> LLVVGPKFIRANQEYTLVISNFNSQLSKVDLLLKLEGETDNGLSVLNVTKMVDVRRNMNRMINFNMPEDLTAGNYKITIDGQRGFSFHKEAELVYLSKSISGLIQVDKPVFKPGDTVNFRVIVLDTELKPPARVKSVYVTIRDPQRNV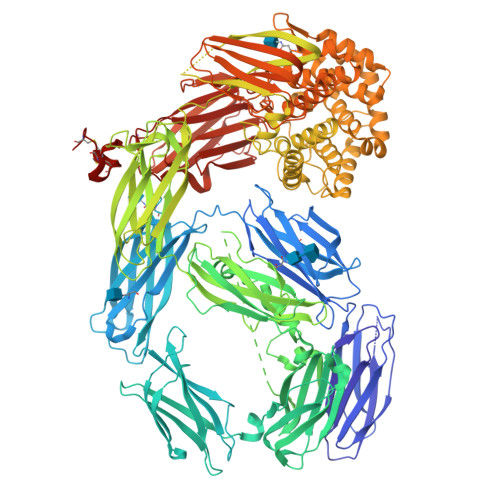IRKWSTAKLYAGVFESDLQIAPTPMLGVWNISVEVEGEELVSKTFEVKEYVLSTFDVQVMPSVIPLEEHQAVNLTIEANYHFGKPVQGVAKVELYLDDDKLKLKKELTVYGKGQVELRFDNFAMDADQQDVPVKVSFVEQYTNRTVVKQSQITVYRYAYRVELIKESPQFRPGLPFKCALQFTHHDGTPAKGISGKVEVSDVRFETTTTSDNDGLIKLELQPSEGTEQLSIHFNAVDGFFFYEDVNKVETVTDAYIKLELKSPIKRNKLMRFMVTCTERMTFFVYYVMSKGNIIDAGFMRPNKQPKYLLQLNATEKMIPRAKILIATVAGRTVVYDFADLDFQELRNNFDLSIDEQEIKPGRQIELSMSGRPGAYVGLAAYDKALLLFNKNHDLFWEDIGQVFDGFHAINENEFDIFHSLGLFARTLDDILFDSANEKTGRNALQSGKPIGKLVSYRTNFQESWLWKNVSIGRSGSRKLIEVVPDTTTSWYLTGFSIDPVYGLGIIKKPIQFTTVQPFYIVENLPYSIKRGEAVVLQFTLFNNLGAEYIADVTLYNVANQTEFVGRPNTDLSYTKSVSVPPKVGVPISFLIKARKLGEMAVRVKASIMLGHETDALEKVIRVMPESLVQPRMDTRFFCFDDHKNQTFPINLDINKKADSGSTKIEFRLNPNLLTTVIKNLDHLLGVPTGCGEQNMVKFVPNILVLDYLHAIGSKEQHLIDKATNLLRQGYQNQMRYRQTDGSFGLWETTNGSVFLTAFVGTSMQTAVKYISDIDAAMVEKALDWLASKQHFSGRFDKAGAEYHKEMQGGLRNGVALTSYVLMALLENDIAKAKHAEVIQKGMTYLSNQFGSINNAYDLSIATYAMMLNGHTMKEEALNKLIDMSFIDADKNERFWNTTNPIETTAYALLSFVMAEKYTDGIPVMNWLVNQRYVTGSFPSTQDTFVGLKALTKMAEKISPSRNDYTVQLKYKKSAKYFKINSEQIDVENFVDIPEDTKKLEINVGGIGFGLLEVVYQFNLNLVNFENRFQLDLEKQNTGSDYELRLKVCASYIPQLTDRRSNMALIEVTLPSGYVVDRNPISEQTKVNPIQKTEIRYGGTSVVLYYDNMGSERNCFTLTAYRRFKVALKRPAYVVVYDYYNTNLNAIKVYEVDKQNLCEICDEEDCPAECGGHHHHHH As a part of efforts to develop new therapeutics and diagnostics for melioidosis, the Seattle Structural Genomics Center for Infectious Disease (SSGCID) has determined the crystal structure of betaine aldehyde dehydrogenase (BADH) from B. pseudomallei (BpBADH). BADH catalyzes the irreversible oxidation of betaine aldehyde to the osmoprotectant betaine and is being investigated as a drug target for drug-resistant bacteria, notably Pseudomonas aeruginosa, because its inhibition blocks choline catabolism and leads to the accumulation of the highly toxic betaine aldehyde. The structure also contains 21 helices, 21 strands, four β-hairpins, four β-bulges and 25 helix–helix interactions. BpBADH has a prototypical BADH topology and shares considerable structure and sequence similarity with the ortholog from P. aeruginosa (PaBADH). The 489 amino acids in each monomer fold as 20.4% β-strand, 39.3% α-helix, 2.5% 310-helix and 37.8% loops, forming six β-α-β motifs that contain five β-sheets (four mixed and one antiparallel).

The monomers are very similar and have an r.m.s.d. of ∼0.17 Å for main-chain atoms. The high-resolution structures of betaine aldehyde dehydro­genase from B. pseudomallei (BpBADH) and P. aeruginosa (PaBADH) reveal a conserved NAD-dependent topology and structural similarity. PaBADH is known to be inhibited by disulfiram through the catalytic cysteine; thus, we hypothesize that BpBADH will likewise be inhibited by disulfiram. Disulfiram binds irreversibly to Cys286 in PaBADH, which is in the highly conserved cofactor-binding cavity of PaBADH and BpBADH; the corresponding residue is Cys285 in BpBADH. Since the key amino-acid residues in inhibitor-binding sites are conserved, the previous studies on PaBADH could facilitate the development of small-molecule inhibitors of BpBADH.

>[2x]MSVYGLQRLYIAGAHADATSGKTFDTFDPATGELLARVQQASADDVDRAVASAREGQREWAAMTAMQRSRILRRAVELLRERNDALAELEMRDTGKPIAETRAVDIVTGADVIEYYAGLATAIEGLQVPLRPESFVYTRREPLGVCAGIGAWNYPIQIACWKSAPALAAGNAMIFKPSEVTPLSALKLAEIYTEAGVPAGVFNVVQGDGSVGALLSAHPGIAKVSFTGGVETGKKVMSLAGASSLKEVTMELGGKSPLIVFDDADLDRAADIAVTANFFSAGQVCTNGTRVFVQQAVKDAFVERVLARVARIRVGKPSDSDTNFGPLASAAQLDKVLGYIDSGKAEGAKLLAGGARLVNDHFASGQYVAPTVFGDCRDDMRIVREEIFGPVMSILSFETEDEAIARANATDYGLAAGVVTENLSRAHRAIHRLEAGICWINTWGESPAEMPVGGYKQSGVGRENGITTLEHYTRIKSVQVELGRYQPVFGHHHHHH>MQNGYTYEDYQDTAKWLLSHTEQRPQVAVICGSGLGGLVNKLTQAQTFDYSEIPNFPE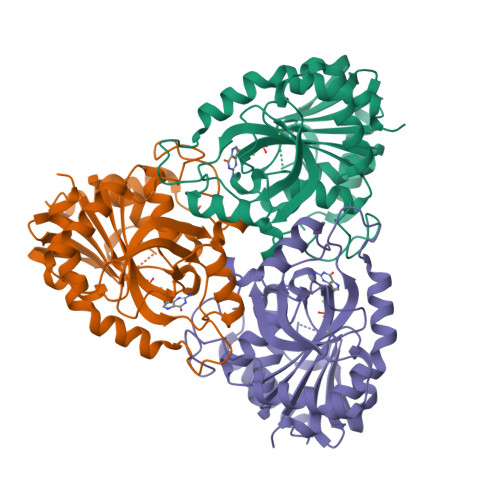STVPGHAGRLVFGILNGRACVMMQGRFHMYEGYPFWKVTFPVRVFRLLGVETLVVTNAAGGLNPNFEVGDIMLIRDHINLPGFSGENPLRGPNEERFGVRFPAMSDAYDRDMRQKAHSTWKQMGEQRELQEGTYVMLGGPNFETVAECRLLRNLGADAVGMSTVPEVIVARHCGLRVFGFSLITNKVIMDYESQGKANHEEVLEAGKQAAQKLEQFVSLLMASIPV[3x]>MRGSHHHHHHMQILLANPRGFCAGVDRAISIVENALAIYGAPIYVRHEVVHNRYVVDSLRERGAIFIEQISEVPDGAILIFSAHGVSQAVRNEAKSRDLTVFDATCPLVTKVHMEVARASRRGEESILIGHAGHPEVEGTMGQYSNPEGGMYLVESPDDVWKLTVKNEEKLSFMTQTTLSVDDTSDVIDALRKRFPKIVGPRKDDICYATTNRQEAVRALAEQAEVVLVVGSKNSSNSNRLAELAQRMGKRAFLIDDAKDIQEEWVKEVKCVGVTAGASAPDILVQNVVARLQQLGGGE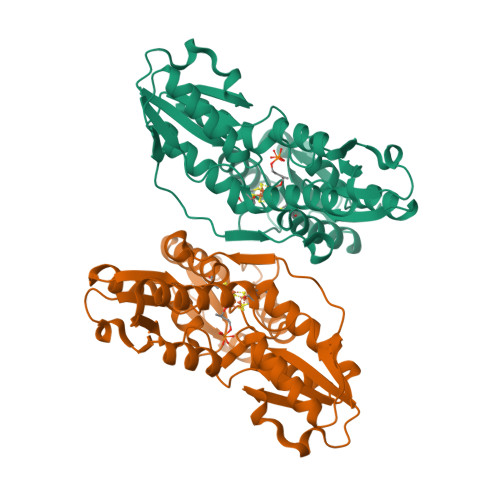AIPLEGREENIVFEVPKELRVDIREVD[2x]> KCPVTHLTTDAGAPVVDNQNSMTAGARGPLLAQDLWLNEKLGNFVREVIPERRMHAKGSGAFGTFTVTHDITQYTRAKLFSEIGKKTDIFVRFSTVAGERGAADAERDIRGFAMKFYTEEGNWDLVGNNTPVFFLRDARKFPDLNKAVKRDPKTNKRSATNNWDFWTLLPEALHQVTIVMSDRGIPDGYRHMHGFGSHTF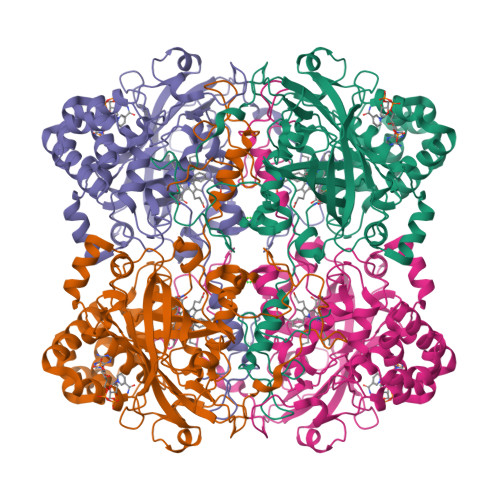SFINANNERFWVKFHMRTQQGIKNLTDAEAEAIIAKDRESSQTDLFDAIERGDFPKWKMYVQIMPELDAEKVPYHPFDLTKVWPKGDYPLIEVGEFELNRNPENYFQDVEQAAFAPSNLVPGISFSPDRMLQARLFNYADAARYRVGVNHYQIPVNAPRCPVHSNRRDGQGRTDGNYGALPHYEPNSFSQWQEQPQYKEPPLKISGAADFWDYREDDNDYFSQPRALFNLMNDQQKQALFDNTAAAMGDALDFIKYRHIRNCYACDPAYGEGVAKALGMTVADAQAARATDPAQGNPGLL>MDNYQELRVQFAAQAVDRNEIEQWVREFAYQGFDARRVIELLKQYGGADWEKDAKKMIVLALTRGNKPRRMMMKMSKEGKATVEALINKYKLKEGNPSRDELTLSRVAAALAGWTCQALVVLSEWLPVTGTTMDGLSPAYPRHMMHPSFAGMVDPSLPGDYLRAILDAHSLYLLQFSRVINPNLRGRTKEEVAATFTQPMNAA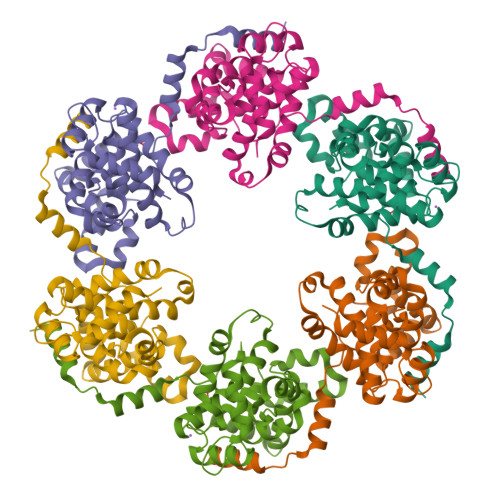VNSNFISHEKRREFLKAFGLVDSNGKPSAAVMAAAQAYKTAA[3x]>MACNKQNGVKNILITFTDCDTQEVIGPISHEQPDDTLPTYKNCAWTNTALTNGYVQRSASNATMTLPVVRDLRVPLAFYQGCAQVDVQVEKFDGTVMTLTEGAVVEPEESDGRSVTMNIVASEIDELLPPGSLAAA[18x];>[12x]MAQDALSDGFVRLCIDPSLNFFGEGCKILVEGQMTDDGSATPDAVTCVTSELDIIERFGQGSVLTESLRKVFCTCKSGVSVYALPREDAAAGVKAVYTLTIAGPATTDGRVQLYMGEAEYAVDIGVDAGDTATDIAAAIVAAISPDFPYAATAAAGVITLTARNAGTIGNHLSVIYTNLGSCTSVTPEGVTVTFAQTTAGSVNPTPNDYATVVNECCFAVYVLSSDDTDWQENLRDWIRSAWDCSKPQCFGHGYVFNKGTLGQVLADGDNSAELSRLALPTTYPVLPYLTNAAYGALSACSTCNNPELNIQGQTFGLLSCINMPESCTPGWTFGEVTQLQANGFVVSGPSTTSGQGNYTSPYIYNDVTNYLRDEKNRPNATFRDASSRRLAAATGVALAEFLQQFNGLAVFTKNTNIRTGIIGTNPRLMLGKIRKWAQDNVGTLFSEFDNINEDIQLLTDFEVQPKCVGQPGIFHLNMRYRPPVRGARIN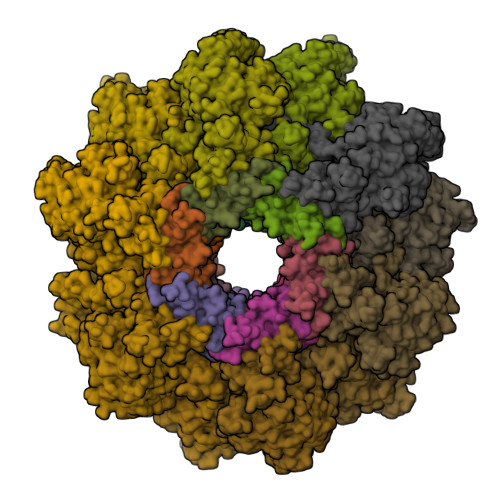VNMAPALFDNCDR>GPMRSRIFKIIVIGDSNVGKTCLTYRFCAGRFPDRTEATIGVDFRERAVEIDGERIKIQLWDTAGLERFRKSMVQHYYRNVHAVVFVYDMTN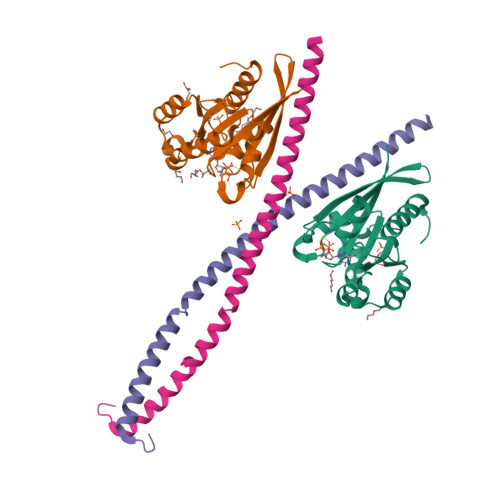MASFHSLPSWIEECKQHLLANDIPRILVGNKCDLRSAIQVPTDLAQKFADTHSMPLFETSAKNPNDNDHVEAIFMTLAHKLKSHKPLMLSQPPDNGIILK[2x];>[2x]MLETNCLDLRTKLQDLEVANQTLKDEYDALQITFTALEEKLRKTTEENQELVTRWMAEKAQEANRLNAENEKDSRRRQARLQKELAEAAKEPLPVEQDDDIEVIVDETSDHTEETSPVRAVSRAAT> MDVTCNIKNGRCEQFCKNSADNKVVCSCTEGYRLAENQKSCEPAVPFPCGRVSVSQTSKLTR;> VVGGEDAKPGQFPWQVVLNGKVDAFCGGSIVNEKWIVTAAHCVETGVKITVVAGEHNIEETEHTEQKRNVIRIIPHHNYNAAINKYNHDIALLELDEPLVLNSYVTPICIADKEYTNIFLKFGSGYVSGWGRVFHQGQSALVLQYLRVPLVDRATCLRS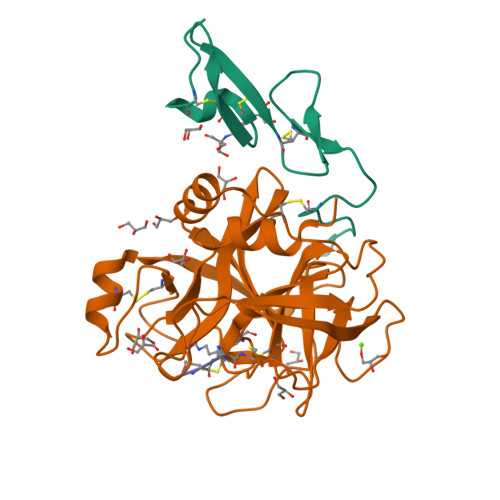TKFTIYNNMFCAGFHEGGRDSCQGDSGGPHVTEVEGTSFLTGIISWGEECAMKGKYGIYTKVSRYVNWIKEKTKLT>MSKSSYYAPHGGHPAQTELLTDRAMFTEAYAVIPKGVMRDIVTSHLPFWDNMRMWVIARPLSGFAETFSQYIVELAPNGGSDKPEQD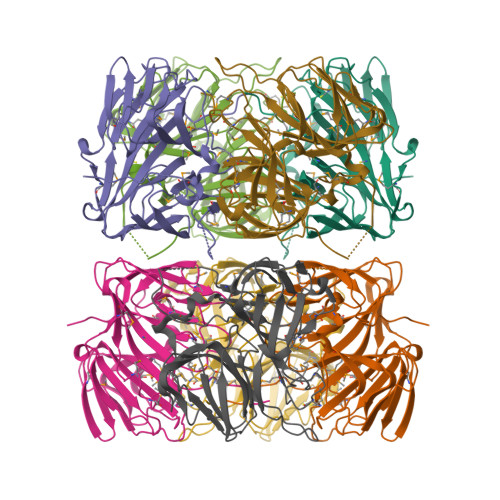PNAEAVLFVVEGELSLTLQGQVHAMQPGGYAFIPPGADYKVRNTTGQHTRFHWIRKHYQKVDGVPLPEAFVTNEQDIQPLVMPDTEGRWSTTRFVDMSDMRHDMHVNIVNFEPGGVIPFAETHVMEHGLYVLEGKAVYRLNQDWVEVEAGDFMWLRAFCPQACYSGGPGRFRYLLYKDVNRHMRLTLNAPH[2x]> MEHLYIVSYDIRNQRRWRRLFKTMHGFGCWLQLSVFQCRLDRIRIIKMEAAINEIVNH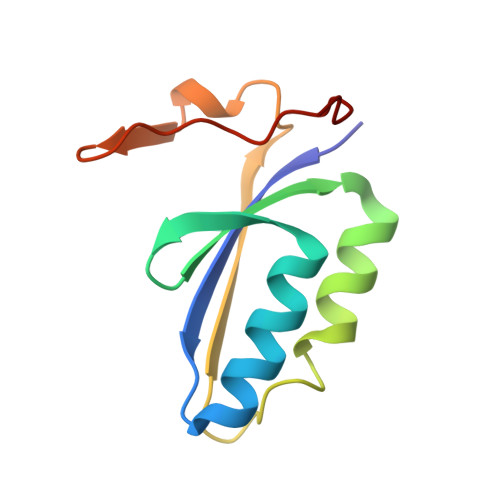AEDHVLILDLGPAENVKPKVSSIGKTFDPILRQAVIV> AGACIDGASLSFDILKTVLEALGNVKRKIAVGVDNESGKTWTALNTYFRSGTSDIVLPHKVPHGCALLYNGQKDRGPVATGAVGVLAYLMSDGNTLAVLFSVPYDYNWYSNWWNVRIYKGKR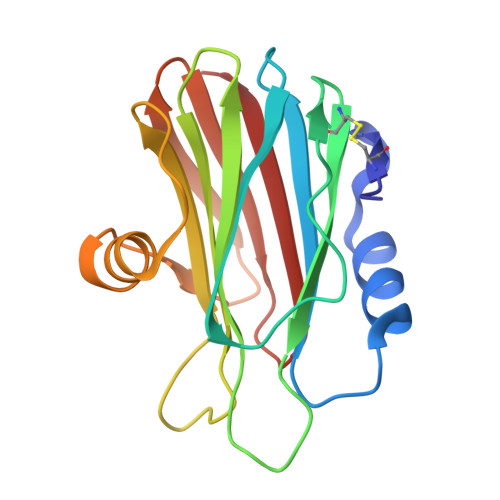RADQRMYEELYYNLSPFRGDNGWHTRNLGYGLKSRGFMNSSGHAILEIHVSKA> DDYLDRLPKSKKGLQGLLQDIEKRILHYKQLFFKEQNEIANGKRSMVPDNSIPICSDVTKLNFQALIDAQMRHAGKMFDVIMMDPPWQLSSSQPSRGVAIAYDSLSDEKIQNMPIQSLQQDGFIFVWAINAKYRVTIKMIENWGYKLVDEITWVKKTVNGKIAKGHGFYLQHAKESCLIGVKGDVDNGRFKKNIASDVIFSERRGQSQKP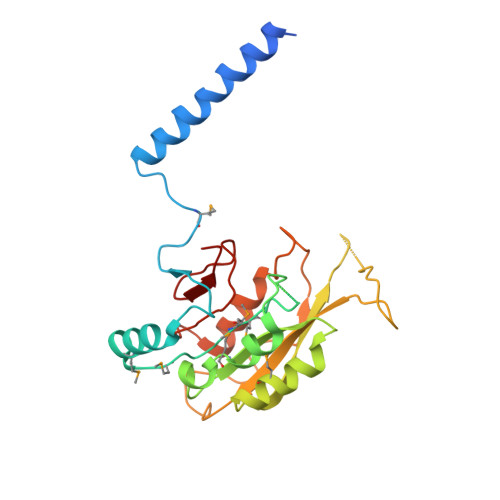EEIYQYINQLCPNGNYLEIFARRNNLHDNWVSIGNEL>[2x]GPLGSAAASFGQTKIPRGNGPYSVGCTDLMFDHTNKGTFLRLYYPSQDNDRLDTLWIPNKEYFWGLSKFLGTHWLMGNILRLLFGSMTTPANWNSPLRPGEKYPLVVFSHGLGAFRTLYSAIGIDLASHGFIVAAVEHRDRSASATYYFKDQSAAEIGDKSWLYLRTLKQEEETHIRNEQVRQRAKECSQALSLILDIDHGKPVKNALDLKFDME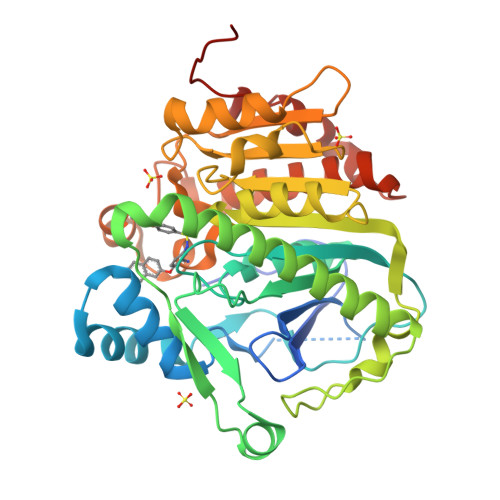QLKDSIDREKIAVIGHSFGGATVIQTLSEDQRFRCGIALDAWMFPLGDEVYSRIPQPLFFINSEYFQYPANIIKMKKCYSPDKERKMITIRGSVHQNFADFTFATGKIIGHMLKLKGDIDSNVAIDLSNKASLAFLQKHLGLHKDFDQWDCLIEGDDENLIPGTNINTTNQHI3-[1-(3-phenylpropyl)-1,2,3,6-tetrahydropyridin-4-yl]-1H-pyrrolo[2,3-b]pyridine 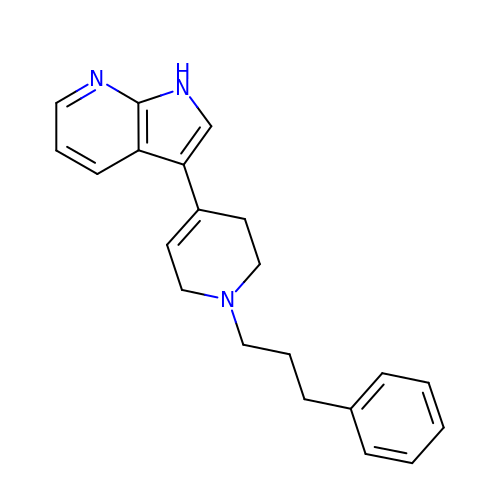| C21 H23 N3 | IWLWNPOFKPUZCM-UHFFFAOYSA-N The photoreceptor archaerhodopsin-3 (AR3) from the archaebacterium Halorubrum sodomense is a light-driven proton transporter. Like other microbial rhodopsins, it has seven transmembrane helices and a retinylidene chromophore created by the covalent conjugation of retinal to Lys226 via a Schiff base. Absorption of a photon of appropriate wavelength initiates a highly ordered sequence of conformational changes (the photocycle) which results in the movement of one H+ ion from the cytoplasm to the extracellular medium. AR3, along with many other microbial rhodopsins, has a desensitized, dark-adapted (DA) state which is formed from the resting, light-adapted (LA) state in the absence of light.

In this study, microcrystals of AR3 were prepared for data collection in light and dark environments by sandwiching them between 13 µm thick sheets of polymer film with high X-ray transmittance. Transparent cyclic olefin polymer (COP) and opaque black Kapton provided light-permissive and light-tight containment, respectively, and enabled diffraction data to be collected at room temperature, significantly reducing the risk of crystal dehydration. The opaque sample mount enabled AR3 desensitization to the DA state, which was maintained and captured at 1.9 Å resolution in the diffraction data. This research not only demonstrates that AR3 can convert from LA to DA in a crystalline environment, but also that conversion to the DA state can take place at room temperature, with no apparent input of energy. The DA state is characterized by a thermal equilibrium between at least two conformations: one possessing all-trans retinal, in common with the LA state, and one with 13-cis 15-syn retinal. All of the key structural features of AR3 were resolved, including the retinal chromophore, which is present as the 13-cis isomer in the DA state and as the all-trans isomer in the LA state. Two different retinal conformers are modelled for each structure and the greatest apparent movement is around the β-ionone ring. Although the room-temperature structures are at lower resolution, the conformations of retinal observed here are broadly consistent with those in the previously reported cryo structures. All of the major structural features visible in the high-resolution cryo crystal structures were also resolved at room temperature, including the retinylidene chromophore, which is formed from the covalent conjugation of retinal to Lys226, and the conversion of the N-terminal Gln7 to a pyroglutamyl group. Arg92, which is resolved as four rotamers in the two cryo structures, is only resolved in one position in the two room-temperature structures.

> QAGYDLLGDGRPETLWLGIGTLLMLIGTFYFLVRGWGVTDKDAREYYAVTILVPGIASAAYLSMFFGIGLTEVTVGGEMLDIYYARYADWLFTTPLLLLDLALLAKVDRVTIGTLVGVDALMIVTGLIGALSHTAIARYSWWLFSTICMIVVLYFLATSLRSAAKERGPEVASTFNTLTALVLVLWTAYPILWIIGTEGAGVVGLGIETLLFMVLDVTAKVGFGFILLRSRAILGDTEAPE Vibrio α-hemolysins (αHLs) are β-pore-forming toxins secreted by Vibrio pathogens, crucial for the facilitation of bacterial infections through host cell lysis. These toxins are produced as inactive precursors, requiring proteolytic maturation and membrane association for activation within host tissues. Here, we investigate Vibrio campbellii αHL (VcαHL), and establish that its hemolytic activity is significantly stimulated by calcium ions, with an EC50 that aligns with physiological calcium concentrations. Using X-ray crystallography and cryo-electron microscopy, we decipher both the immature and assembled structures of VcαHL and elucidate the conformational changes corresponding to toxin assembly.

To further explore the mechanism of calcium-mediated stimulation of VcαHL, we determined the crystal structure of pro-VcαHL. Paralleling the structure of pro-VCC, this structure also shows four distinct domains: a pro domain, a cytolysin domain, a β-trefoil lectin domain, and a β-prism lectin domain. However, the β-prism lectin domain of pro-VcαHL is situated at a distinct position, forming a unique conformation. In pro-VcαHL, the β-prism lectin domain primarily interacts with the β-trefoil lectin domain, contrasting with its binding to the pre-stem loop in the pro-VCC structure. Several hydrogen bonds and salt bridges were formed between the β-prism and β-trefoil lectin domains, stabilizing the domain interactions in pro-VcαHL. In addition, the pre-stem loop in pro-VcαHL interacts with the β-trefoil lectin and cytolysin domains through several polar interactions. Two lysine residues, K300 and K302, interact with the β-trefoil lectin domain through side-chain associations with T534 and E529, respectively. Multiple residues at the interface between the pre-stem loop and the cytolysin domain engage in the formation of hydrogen bonds and salt bridges. In pro-VcαHL, H137 forms a hydrogen bond with a sulfate ion that binds to R313 of the pre-stem loop, while E185 participates in interactions with Q311 on the pre-stem loop. This sulfate ion forms a hydrogen bond network with water molecules, connecting E95 of pro domain and N183 of cytolysin domain in pro-VcαHL.

> MNINEPSGEAANIISQAADSHAMKYYNAADWQAEDNALPSLAELRDLVINQQKSVLFDFSQNSDADGQAEMQAQFRKTYGVGFANQFIFITEHKGELLFTPFEHSEEVDPKLLEAPLTTRSGLKSTAPTNSETSTLPHVAFYISVNRPISDEECTFDNSWLWKDEKGSRPFCKDANISLIYRVNLERSLQYGIVGSATPNAKIVRISLDDDSSGAGIHLNDQLSYRRFGASYTTLDAYFREWSTDAIAQDYRFVFKTSNNKAEILETFPIDNLNVKYEKRKQSGFELGVTGGAEVSEDGPKAKLEARASITQSRWLTYNTQDYRVERNAKNAQTVSFTWNRQEYATAESLLNRSTDALWVDTYPVDVNRISPLSYASFVPKMDVIYKASDTETGSTDFIIDSSVNIRPIYNGAYKHYYVVGAHQSYHGFENSPRRRITKSASFTVDWDHPVFTGGRPVNLQLASFNNRCVQVDAQSRLTANTCDDQQSAQSFIYDQLGRYVSASNTELCLDGAALDVLQTCNQNLTQRWEWRKNTDELTNVYSGESLGHDKQTGELGLYASSNDAVSLRTITAYTNVFNVQKSSPILGYTQGKMNQQSVGQNYRLYVREGSAIDALGTASDLLVGGNGGSLTSVDLSGVKSITATSGDFQYGGQQLVALTFTYQDGRQQMVGSKAHVTNAHEDRFDLPDAAKITQLNIWADDWLVKGVQFDLNLEHHHHHH> HMGSDTDERSAALDAEEMATRARAASNLLKALAHEGRLMIMCYLASGEKSVTELE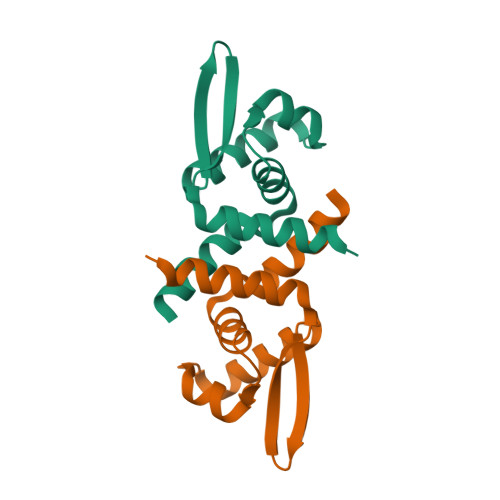TRLSTRQAAVSQQLARLRLEGLVQSRREGKTIYYSLSDPRAARVVQTVYEQFCSGD>GSSHHHHHHSSGENLYFQGHMTCPFADPAALYSRQDTTSGQSPLAAYEVDDSTGYLTSDVGGPIQDQTSLKAGIRGPTLLEDFMFRQKIQHFDHERVPERAVHARGAGAHGTFTSYADWSNITAASFLNATGKQTPVFVRFSTCAGSRGSADTARDVHGFATRFYTDEGNFDIVGNNIPVFFIQDAIQFPDLIHSVKPRPDNEIPQAATAHDSAWDFFSQQPSTMHTLFWAMSGHGIPRSYRHMDGFGVHTFRFVKDDGSSKLIKWHFKSRQGKASLVWEEAQVLSGKNADFHRQDLWDAIESGNGPEWDVCVQIVDESQAQAFGFDLLDPT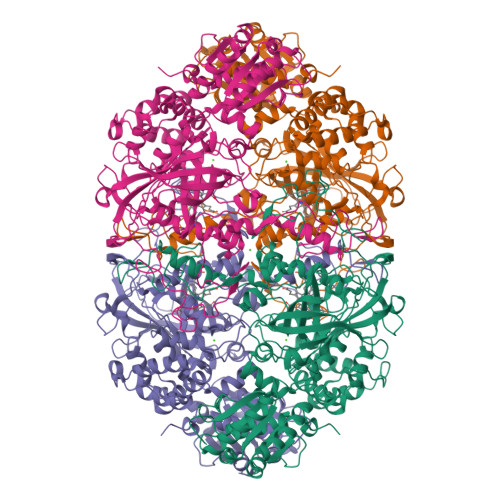KIIPEEYAPLTKLGLLKLDRNPTNYFAETEQVMFQPGHIVRGIDFTEDPLLQGRLFSYLDTQLNRNGGPNFEQLPINMPRVPIHNNNRDGAGQMFIHRNKYPYTPNTLNSGYPRQANQNAGRGFFTAPGRTASGALVREVSPTFNDHWSQPRLFFNSLTPVEQQFLVNAMRFEISLVKSEEVKKNVLTQLNRVSHDVAVRVAAAIGLGAPDADDTYYHNNKTAGVSIVGSGPLPTIKTLRVGILATTSESSALDQAAQLRTRLEKDGLVVTVVAETLREGVDQTYSTADATGFDGVVVVDGAAALFASTASSPLFPTGRPLQIFVDAYRWGKPVGVCGGKSSEVLDAADVPEDGDGVYSEESVDMFVEEFEKGLATFRFTDRFALDS[4x]> MSRPRRRGRDINGVLLLDKPQGMSSNDALQKVKRIYNANRAGHTGALDPLATGMLPICLGEATKFSQYLL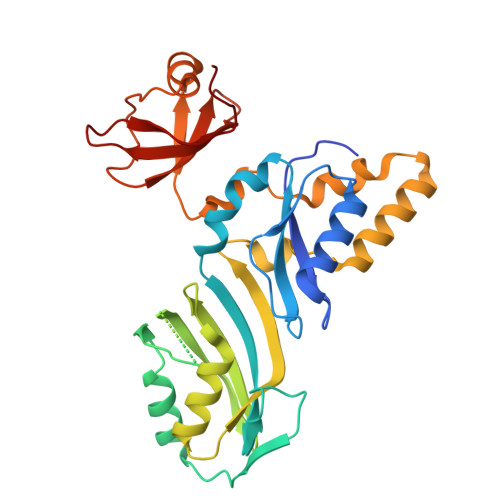DSDKRYRVIARLGQRTDTSDADGQIVEERPVTFSAEQLAAALDTFRGDIEQIPSMYSALKYQGKKLYEYARQGIEVPREARPITVYELLFIRHEGNELELEIHCSKGTYIRTIIDDLGEKLGCGAHVIYLRRLAVSKYPVERMVTLEHLRELVEQAEQQDIPAAELLDPLLMPMDSPASDYPVVNLPLTSSVYFKNGNPVRTSGAPLEGLVRVTEGENGKFIGMGEIDDEGRVAPRRLVVEYPA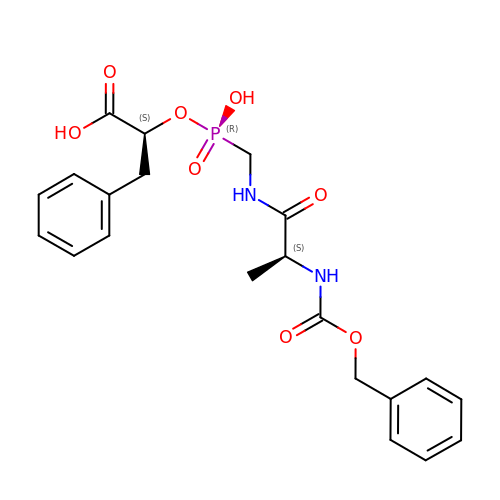O-(((1R)-((N-(PHENYL-METHOXY-CARBONYL)-ALANYL)-AMINO)METHYL)HYDROXYPHOSPHINYL)3-L-PHENYLLACTATE | C21 H25 N2 O8 P | ICACWKLCNCPHAM-YJBOKZPZSA-N>[4x]GS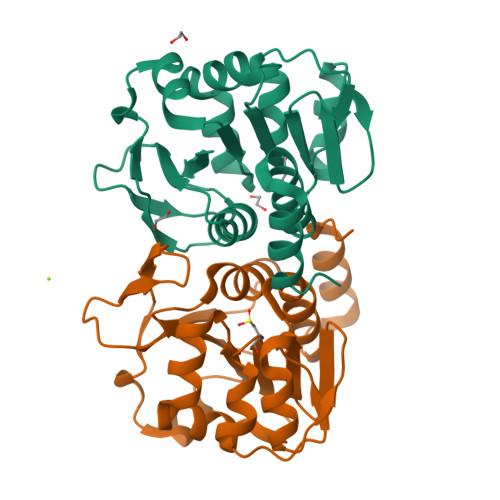HMVKVCLFVADGTDEIEFSAPWGIFKRAEIPIDSVYVGENKDRLVKMSRDVEMYANRSYKEIPSADDFAKQYDIAIIPGGGLGAKTLSTTPFVQQVVKEFYKKPNKWIGMICAGTLTAKTSGLPNKQITGHPSVRGQLEEGGYKYLDQPVVLEENLITSQGPGTAMLFGLKLLEQVASKDKYNAVYKSLSMP> MIESLADWSIFTDPDVFGEPVTWTTPPLPDPVPAIFTDASEDRPATLGPGVLTIAPTLTLGAAQLPFSPARNHRC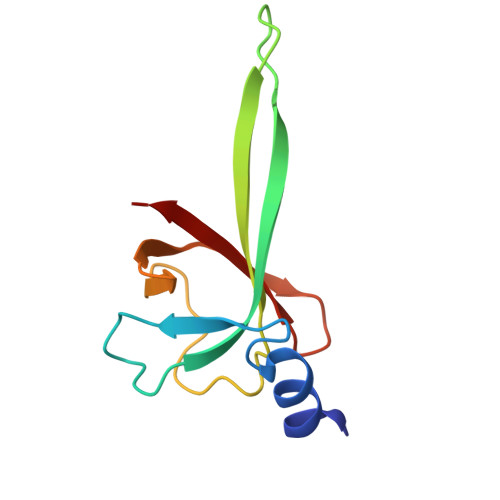TVRGITYRVAEVQPDGSGGLRLLLERV> GSLVDDKVLVSELIGVDPNPFTQRIMIDKGENDGVFVGQPVLDASGLMGQVVEVMPYTARVLLLTDTTHSIPVQVNRNGLRAIAVGTGNPERLELRYVADTADIKEGDLLVSSGLGQRFPAGYPVATVKEVIHDSGQPFAVVRAVPTAKMNRSRYVLLVFSDSR

The elongasome, or Rod system, is a protein complex that controls cell wall formation in rod-shaped bacteria. MreC is a membrane-associated elongasome component that co-localizes with the cytoskeletal element MreB and regulates the activity of cell wall biosynthesis enzymes, in a process that may be dependent on MreC self-association. MreC is a bitopic protein that harbors a large periplasmic domain, whose most noteworthy characteristic is a β−sandwich core reminiscent of ‘butterfly wings’. MreC is essential for shape maintenance in rod-shaped bacteria, and mreC knockout mutants are not viable.

In order to allow unambiguous tracing of the MreCPa structure into the cryo-EM Coulomb potential map, we solved the high-resolution crystal structure of MreCPa(97-258) that harbors only the central β-sandwich core region. Fitting the refined crystallographic model of MreCPa(97-258) into the cryo-EM map confirmed that within each protofilament, monomers are ordered in a polar, head-to-tail fashion, with the β-sandwich folds contributing with complementing charged regions towards formation of the interface between two protofilaments.>MTKIITSPSKFIQGPDELSRLSAYTERLGKKAFIIADDFVTGLVGKTVEESYAGKETGYQMALFGGECSKPEIERLCEMSKSEEADVVVGIGGGKTLDTAKAVGYYNNIPVIVAPTIASTNAPTSALSVIYKENGEFEEYLMLPLNPTFVIMDTKVIASAPARLLVSGMGDALATYFEARATKRANKTTMAGGRVTEAAIALAKLCYDTQILEGLKAKLAAEKHLVTEAVEKIIEANTYLSGIGSESGGLAAAHAIHNGLTVLEETHHMYHGEKVAFGTLAQLILEDAPKAEIEEVVSFCL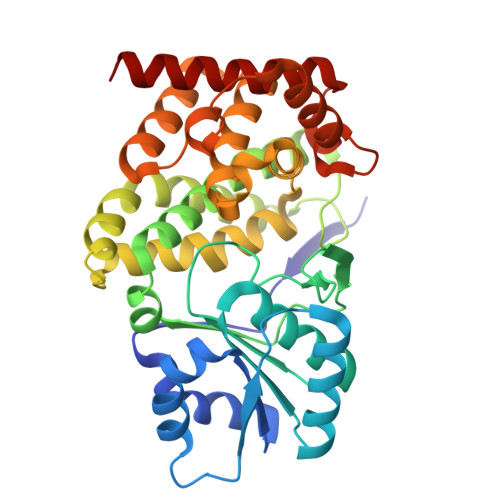SVGLPVTLGDLGVKELNEEKLRKVAELSCAEGETIYNMPFEVTPDLVYAAIVTADSVGRYYKEKW[8x]> MVSNASALGRNGVHDFILVRATAIVLTLYIIYMVGFFATSGELTYEVWIGFFASAFTKVFTLLALFSILIMAWIGMWQVLTDY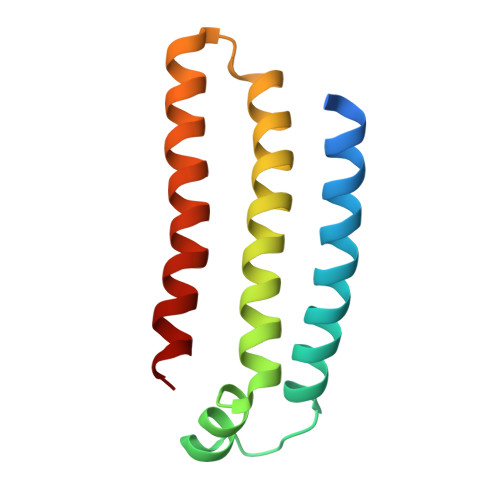VKPLALRLMLQLVIVVALVVYVIYGFVVVWGV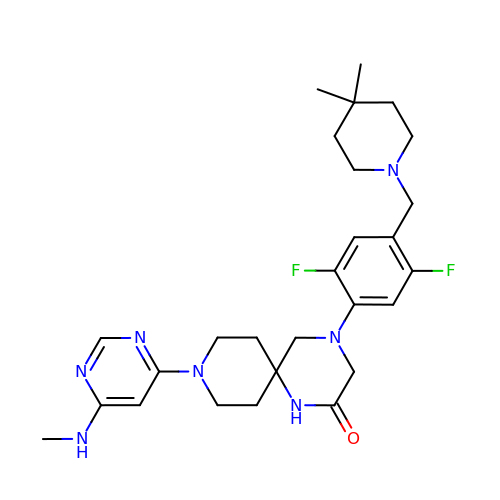4-[4-[(4,4-dimethylpiperidin-1-yl)methyl]-2,5-bis(fluoranyl)phenyl]-9-[6-(methylamino)pyrimidin-4-yl]-1,4,9-triazaspiro[5.5]undecan-2-one | C27 H37 F2 N7 O | GYWOVBUGFWWSJR-UHFFFAOYSA-N>MNKIIIYTDGGARGNPGPAGIGVVITDEKGNTLHESSAYIGETTNNVAEYEALIRALEDLQMFGDKLVDMEVEVRMDSELIVRQMQGVYKVKEPTLKEKFAKIAHIKMERVPNLVFVHIPREKNARADELVNE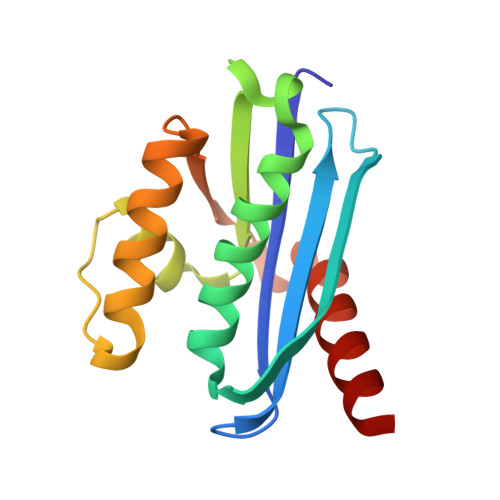AIDKALS[4x]>[2x]AEAGITGTWYAQLGDTFIVTAGADGALTGTYEAAVGNAESRYVLTGRYDSAPATDGSGTALGWTVAWKNNYRNAHSATTWSGQYVGGAEARINTQWLLTSGT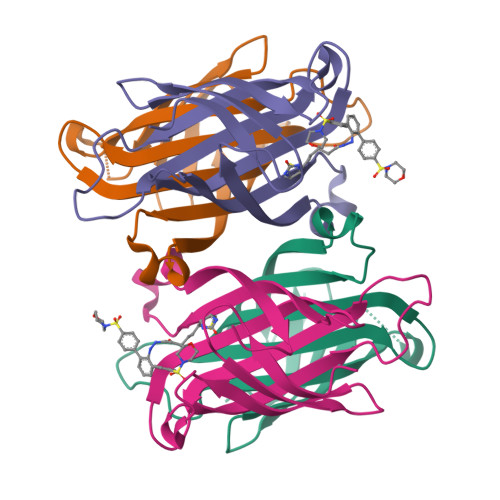TEANAWKSTLVGHDTFTKVKPSAAS;>[2x]AEAGITGTWYNQLGSTFIVTAGADGALTGTYESAVGNAESRYVLTGRYDSAPATDGSGTALGWTVAWKNNYRNAHSATTWSGQYVGGAEARINTQWLLTSGTTEANAWKSTLVGHDTFTKVKPSAASEEEEEE> GGDPHMMFGKKKNNGGSSTARYSAGNKYNTLSNNYALSAQQLLNASKIDDIDSMMGFERYVPPQYNGRFDAKDIDQIPGRVGWLTNMHATLVSQETLSSGSNGGGNSNDGERVTTNQGISGVDFYFLDEEGGSFKSTVVYDPYFFIACNDESRVNDVEELVKKYLESCLKSLQIIRKEDLTMDNHLLGLQKTLIKLSFVNSNQLFEARKLLRPILQDNANNNVQRNIYNVAANGSEKVDAKHLIEDIREYDVPYHVRVSIDKDIRVGKWYKVTQQGFIEDTRKIAFADPVVMAFAIATTKPPLKFPDSAVDQIMMISYMIDGEGFLITNREIISEDIEDFEYTPKPEYPGFFTIFNENDEVALLQRFFEHIRDVRPTVISTFNGDFFDWPFIHNRSKIHGLDMFDEIGFAPDAEGEYKSSYCSHMDCFRWVKRDSYLPQGSQGLKAVTQSKLGYNPIELDPELMTPYAFEKPQHLSEYSVSDAVATYYLYMKYVHPFIFSLCTIIPLNPDETLRKGTGTLCEMLLMVQAYQHNILLPNKHTDPIERFYDGHLLESETYVGGHVESLEAGVFRSDLKNEFKIDPSAIDELLQELPEALKFSVEVENKSSVDKVTNFEEIKNQITQKLLELKENNIRNELPLIYHVDVASMYPNIMTTNRLQPDSIKAERDCASCDFNRPGKTCARKLKWAWRGEFFPSKMDEYNMIKRALQNETFPNKNKFSKKKVLTFDELSYADQVIHIKKRLTEYSRKVYHRVKVSEIVEREAIVCQRENPFYVDTVKSFRDRRYEFKGLAKTWKGNLSKIDPSDKHARDEAKKMIVLYDSLQLAHKVILNSFYGYVMRKGSRWYSMEMAGITCLTGATIIQMARALVERVGRPLELDTDGIWCILPKSFPETYFFTLENGKKLYLSYPCSMLNYRVHQKFTNHQYQELKDPLNYIYETHSENTIFFEVDGPYKAMILPSSKEEGKGIKKRYAVFNEDGSLAELKGFELKRRGELQLIKNFQSDIFKVFLE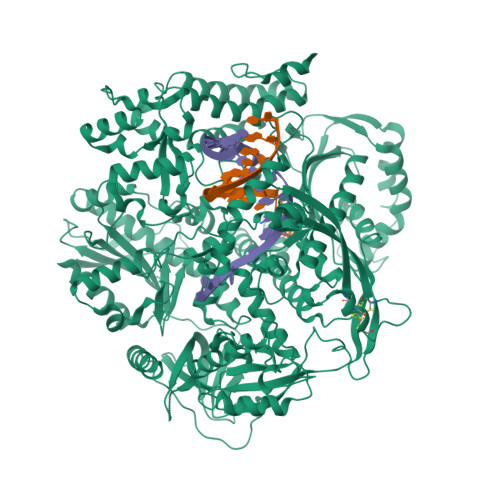GDTLEGCYSAVASVCNRWLDVLDSHGLMLEDEDLVSLICENRSMSKTLKEYEGQKSTSITTARRLGDFLGEDMVKDKGLQCKYIISSKPFNAPVTERAIPVAIFSADIPIKRSFLRRWTLDPSLEDLDIRTIIDWGYYRERLGSAIQKIITIPAALQGVSNPVPRVEHPDWLKRKIATK>[4x]MENLISLVNKIQRACTALGDHGDSSALPTLWDSLPAIAVVGGQSSGKSSVLESIVGKDFLPRGSGIVTRRPLVLQLQKIDDGTREYAEFLHLPRKKFTDFAAVRKEIQDETDRETGRSKAISSVPIHLSIYSP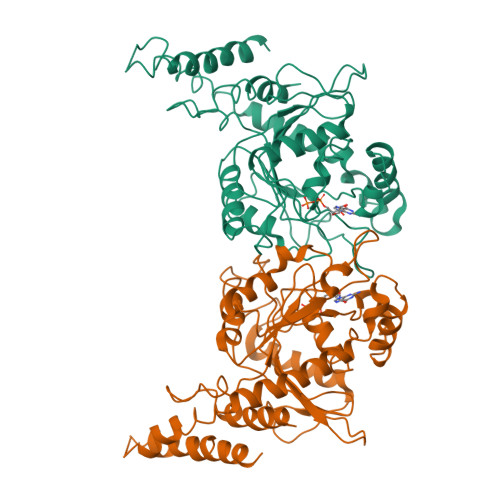NVVNLTLIDLPGLTKVAVDGQSDSIVKDIENMVRSYIEKPNCIILAISPANQDLATSDAIKISREVDPSGDRTFGVLTKIDLMDKGTDAVEILEGRSFKLKYPWVGVVNRSQADINKNVDMIAARKREREYFSNTTEYRHLANKMGSEHLAKMLSKHLERVIKSRIPGIQSLINKTVLELETELSRLGKPIAHGTDSRVDPAIMERRSAISKRLELYRAAQSEIDAV> MTYKLYIMTFQNAHFGSGTLDSSKLTFSADRIFSALVLESLKMGKLDAFLAEANQDKFTLTDAFPFQFGPFLPKPIGYPKHDQIDQSVDVKEVRRQAKLSKKLQFLALENVDDYLNGELFENEEHAVIDTVTKNQPHKDGNLYQVATTRFSNDTSLYVIANESDLLNELMSSLQYSGLGGKRSSGFGRFEL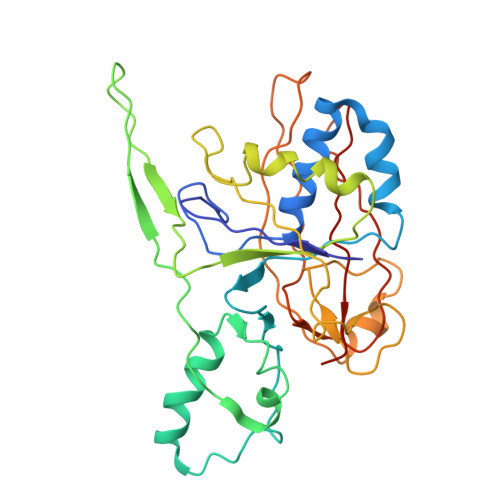DIQNIPLELSDRLTKNHSDKVMSLTTALPVDADLEEAMEDGHYLLTKSSGFAFSHATNENYRKQDLYKFASGSTFSKTFEGQIVDVRPLDFPHAVLNYAKPLFFKLEV>[2x]IQTTAPPVKESSFVEKMKKTGRNIIVFYGSQTGTAEEFANRLSKDAHRYGMRGMSADPEEYDLADLSSLPEIDKSLVVFCMATYGEGDPTDNAQDFYDWLQETDVDLTGVKFAVFGLGNKTYEHFNAMGKYVDQRLEQLGAQRIFELGLGDDDGNLEEDFITWREQFWPAVCEFFGVEATGEESSIRQYELVVHEDMDVAKVYTGEMGRLKSYENQKPPFDAKNPFLAAVTANRKLNQGTERHLMHLELDISDSKIRYESGDHVAVYPANDSALVNQIGEILGADLDVIMSLNNLDEESNKKHPFPCPTTYRTALTYYLDITNPPRTNVLYELAQYASEPSEQEHLHKMASSSGEGKELYLSWVVEARRHILAILQDYPSLRPPIDHLCELLPRLQARYYSIASSSK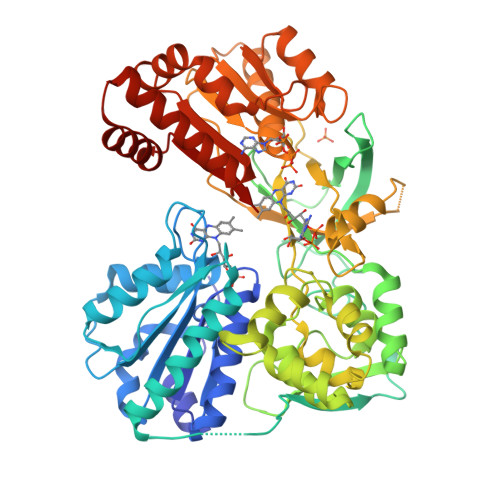VHPNSVHICAVAVEYEAKSGRVNKGVATSWLRAKEPAGENGGRALVPMFVRKSQFRLPFKSTTPVIMVGPGTGIAPFMGFIQERAWLREQGKEVGETLLYYGCRRSDEDYLYREELARFHKDGALTQLNVAFSREQAHKVYVQHLLKRDREHLWKLIHEGGAHIYVCGDARNMAKDVQNTFYDIVAEFGPMEHTQAVDYVKKLMTKGRYSLDVWS> MENTENSVDSKSIKNLEPKIIHGSESMDSGISLDNSYKMDYPEMGLCIIINNKNFHKSTGMTSRSGTDVDAANLRETFRNLKYEVRNKNDLTREEIVEL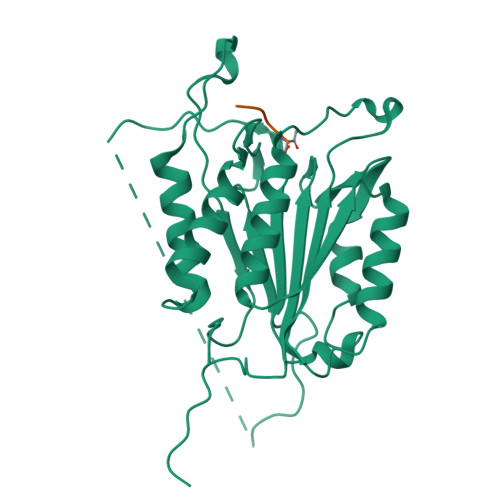MRDVSKEDHSKRSSFVCVLLSHGEEGIIFGTNGPVDLKKITNFFRGDRCRSLTGKPKLFIIQACRGTELDCGIETDSGVDDDMACHKIPVEADFLYACSTAPGYYSWRNSKDGSWFIQSLCAMLKQYADKLEFMHILTRVNRKVATEFESFSFDATFHAKKQIPCIHSMLTKELYFYH> SGCPQRSCKTHVLLLVLHGGNILDTGAGDPSCKAADIHTFSSVLEKVTRAHFPAALGHILIKFVPCPAICSEAFSLVSHLNPYSHDEGCLSSSQDHVPLAALPLLAISSPQYQDAVATVIERANQVYREFLKSSDGIGFSGQVCLIGDCVGGLLAFDAICY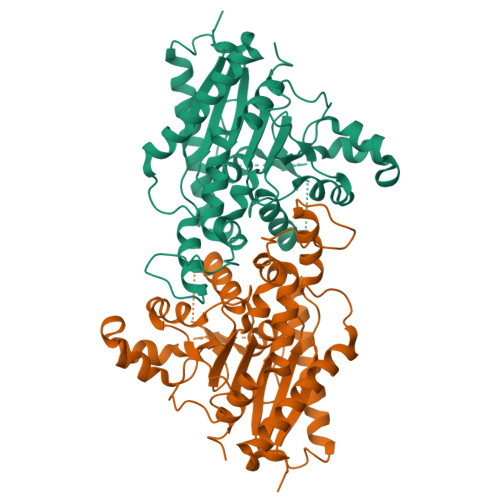SAGPSGDSSDSSTYDCEAITQHHAFLSSIHSSVLKDESETPAAGGPQLPEVSLGRFDFDVSDFFLFGSPLGLVLAMRRTVLPGLDGFQVRPACSQVYSFFHCADPSASRLEPLLEPKFHLVPPVSVPRYQRFPLGDGQSLLLADALHTHSPLFLEGSSDSMAPVGASRITAKWWGSKRIDYALYCPDVLTAFPTVALPHLFHASYWESTDVVAFILRQVMRYESVNIKESA> EDVVWRWSCDNGKCVKLKNDPRSSEPALSLEACKMFCNEYGLLWPRPTGEADLGNFLSKINLNSIEVKILKKGATDDLMEAAAKRFKEQVSLAIPRGSTPKLTGKAVDVYLVNENPNEKAFSLEMDESYGLRVSPSGADRVNATITANSFFGMRHGLETLSQLFVFDDIRDHLLMVRDVNISDKPVYPYRGILLDTARNYYSIESIKRTIEAMAAVKLNTDHWHITDSQSFPFVTTKRPNLYKFGALSPQKVYTKAAIREVVRFGLERGVRVLPEFDAPAHVGEGWQDTDLTVCFKAEPWKSYCVEPPCGQLNPTKDELYQYLEDIYSDMAEVFDTTDIFHMGGDEVSEACWNSSDSIQNFMMQNRWDLDKESFLKLWNYFQQKAQDKAYKAFGKKLPLILWTSTLTNYKHIDDYLNKDDYIIQVWTTGVDPQIKGLLEKGYRLIMSNYDALYFDCGYGAWVGAGNNWCSPYIGWQKVYDNSPAVIALEHRDQVLGGEAALWSEQSDTSTLDGRLWPRAAALAERLWAEPATSWQDAEYRML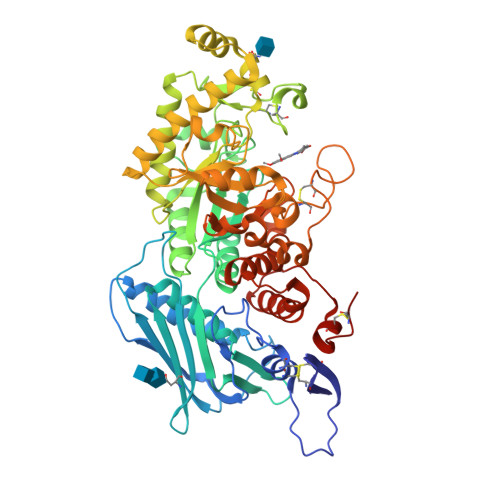HIRERFVRMGIQAESLQPEWCYQNEGYCYSHHHHHH>LNSVGQGEFGGAPFKRFLRGTRIVSGGKLKRMTREKAKQVTVAGVPMPRDAEPRHLLVNGATGTGKSVLLRELAYTGLLRGDRMVIVDPNGDMLSKFGRDKDIILNPYDQRTKGWSFFNEIRNDYDWQRYALSVVPRGKTDEAEEWASYGRLLLRETAKKLALIGTPSMRELFHWTTIATFDDLRGFLEGTLAESLFAGSNEASKALTSARFVLSDKLPEHVTMPDGDFSIRSWLEDPNGGNLFITWREDMGPALRPLISAWVDVVCTSILSLPEEPKRRLWLFIDELASLEKLASLADALTKGRKAGLRVVAGLQSTSQLDDVYGVKEAQTLRASFRSLVVLGGSRTDPKTNEDMSLSLGEHEVERDRYSKNTGKHHSTGRALERVRERVVMPAEIANLP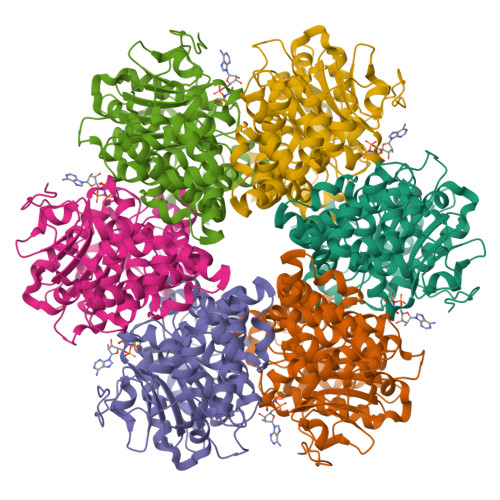DLTAYVGFAGNRPIAKVPLEIKQFANRQPAFVEGTI[6x]>[4x]MELIRFSISIPSKLLEKFDQIIEEIGYENRSEAIRDLIRDFIIRHEWEVGNEEVAGTITIVYNHDEGDVVKALLDLQHEYLDEIIS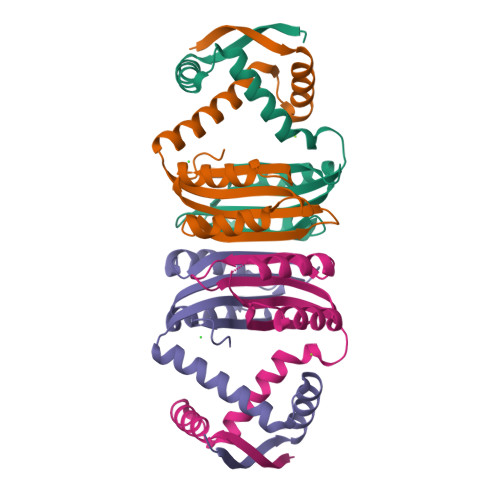SLHVHMDEHNCLEVIVVKGEAKKIKMIADKLLSLKGVKHGKLVMTSTGKELV>[2x]MVVLMTKPGTSDFVWNGIPLSMELNLWNIKEYSGSVAMKFDGEKITFDADIQNLSPKEPERYVLGYPEFYYGYKPWENHTAEGSKLPVPVSSMKSFSVEVS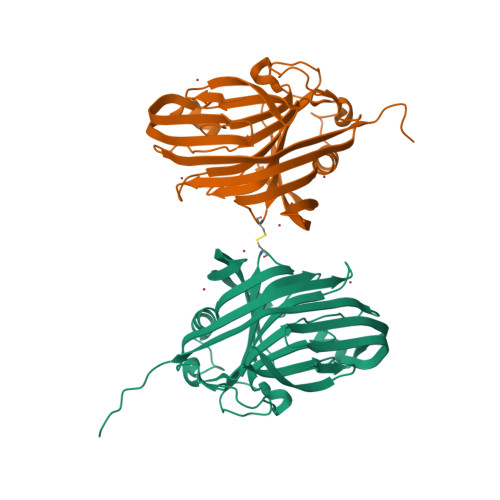FDIHHEPSLPLNFAMETWLTREKYQTEASIGDVEIMVWFYFNNLTPGGEKIEEFTIPFVLNGESVEGTWELWLAEWGWDYLAFRLKCPVKKGRVKFDVRHFLDAAGKALSSSARVKDFEDLYFTVWEIGTEFGSPETKSAQFGWKFENFSIDLEVREHHHHHH> MHHHHHHGSEEQEKALNFGIISTESQQNLKPQWTPFLQDMEKKLGVKVNAFFAPDYAGIIQGMRFNKVDIAWYGNLSAMEAVDRANGQVFAQTVAADGSPGYWSVLIVNKDSPINNLNDLLAKRKDLTFGNGDPNSTSGFLVPGYYVFAKNNISASDFKRTVNAGAETNALAVANKQVDVATNNTENLDKLKTSAPEKLKELKVIWKSPLIPGDPIVWRKNLSETTKDKIYDFFMNYGKTPEEKAVLERLGWAPFRASSDLQLVPIRQLALFKEMQSVKDNKGLNEQDKLAKTTAIQAQLDD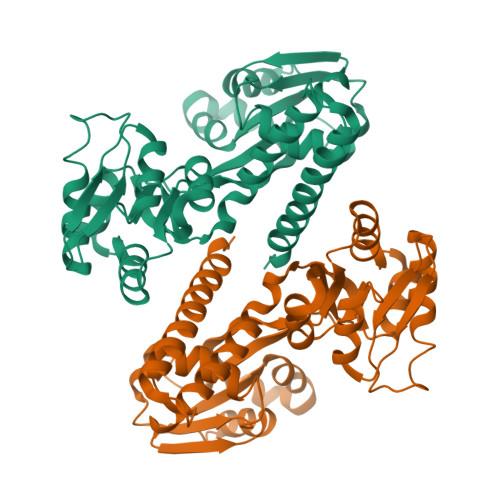LDRLNNALSAMSSVSKAVQ AARSs play an essential role in protein synthesis by charging tRNAs with their cognate amino acids. Similar to other LeuRSs, the C. muris LeuRS contains a predicted editing domain exhibiting highly conserved motifs that are important for the hydrolysis of tRNALeu mischarged with noncognate amino acids, such as isoleucine or norvaline, while excluding cognate Leu-tRNALeu. The structures show the typical seven-β-strand and three-α-helix fold of the LeuRS connective polypeptide domain (CP1), plus archaeon/eukaryote-specific insertions, denoted I1ae, I2ae, I3ae, and I4ae.

Since posttransfer editing by LeuRS in apicomplexans has not been characterized, we performed binding experiments with the CmLeuRS editing domain and posttransfer editing substrate analogues for norvaline, 2-(l-norvalyl)amino-2-deoxyadenosine (Nva2AA), and isoleucine, 2-(l-isoleucyl)amino-2-deoxyadenosine (Ile2AA), which mimic a mischarged amino acid attached to Ade76. Calorimetric titrations yielded dissociation constants (Kds) of 213 and 215 μM for Nva2AA and Ile2AA, respectively, over the range of affinities observed for bacterial LeuRS, but they were lower than those seen for other editing tRNA synthetases, such as class II threonine-tRNA synthetase (ThrRS). These data, together with the conservation of important active-site residues, suggest that CmLeuRS preserves posttransfer editing activity. The posttransfer editing substrate analogues Nva2AA and Ile2AA can be unambiguously placed at the editing site of CmLeuRS. As was observed for bacterial and fungal LeuRSs, the aliphatic part of the amino acid binds into the hydrophobic pocket formed by residues T292 and V426, while the amino group interacts with the universally conserved aspartic acid (D433); the adenine base is accommodated by residues of the GTG loop (I414, S415, V423, and K418). In our structures, a water molecule is well positioned for promoting hydrolysis (3 to 4 Å to the carbon alpha atom) and is coordinated by a eukaryote-specific lysine (K496). A similarly placed water molecule is important for bacterial LeuRS editing complexes, although this is coordinated by a bacterium-specific aspartic acid (D344 in the Thermus thermophilus LeuRS). This suggests a common editing mechanism via nucleophilic attack of this water on the oxygen carbonyl, consistent with quantum mechanical calculations on LeuRS. The interactions of the catalytic water and K496 at the editing site of CmLeuRS are strikingly similar to the situation in the ThrRS-Ser3AA complex, which suggests that K496 could have a similar role in hydrolysis by eukaryotic LeuRS. Compared to the structure of the CmLeuRS-AN6426-AMP complex, the posttransfer analogues retain 3 to 4 extra water molecules (depending on the monomer chain) and a phosphate (CmLeuRS-Ile2AA complex), which mediate polar interactions between the compounds and protein residues.

>[4x]GAMGGPQEYTLIKLKIHLIPEFLGSIVKGREVFVVCATLRPETMYGQTNCWILPDGEYDLVLAFDQVIPYDAKTSDGVLCKIFDKYEDTMKECNTVYICSERSAYNMAYQGIVPLIHGREQGVSDKLLPRIVSLGKVYGEQLIGTPLSAPMTPYSLIFILPMFSISMEKGTGIVTSVPSDSPDDYAALRDIKTKPLLREKYSIKDEWILDPLEIIEVPGFGFMTAELLCNQYKIQSQNDSAKLKQAKEEIYKKEFYEGILIRGKYSGMKICDAKELIRESLIKDGYALIYLE>[2x]DRWGSELPAQKWWHTGALYRIGDLQAFQGHGAGNLAGLKGRLDYLSSLKVKGLVLGPIHKNQKDDVAQTDLLQIDPNFGSKEDFDSLLQ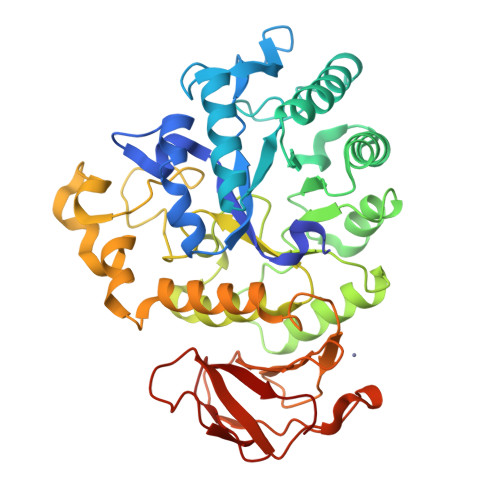SAKKKSIRVILDLTPNYRGENSWFSTQVDTVATKVKDALEFWLQAGVDGFQVRDIENLKDASSFLAEWQNITKGFSEDRLLIAGTNSSDLQQILSLLESNKDLLLTSSYLSDSGSTGEHTKSLVTQYLNATGNRWCSWSLSQARLLTSFLPAQLLRLYQLMLFTLPGTPVFSYGDEIGLDAAALPGQPMEAPVMLWDESSFPDIPGAVSANMTVKGQSEDPGSLLSLFRRLSDQRSKERSLLHGDFHAFSAGPGLFSYIRHWDQNERFLVVLNFGDVGLSAGLQASDLPASASLPAKADLLLSTQPGREEGSPLELERLKLEPHEGLLLRFPYAA>MTTVSEQANFTFSPEEVARFERDGYIGPVKIFEPEEMTRRWNIIRRQLLDRSLAIYPDSNGKANISNYDRHLDIDLLAEHIMRPEIVDRVGSLIGRNLLCWRSEFFPKYQGDEGTDWHQAATFAHATGKPQIIWPSDEGRPAFIGTITVWTAFTHSTEQNGCLQLMPGTHTSMNYDESKGMDYDADAINQREKDGIKRGFFGYDYRSLQKDPDWKPDESQAYPMVLKPGEAVI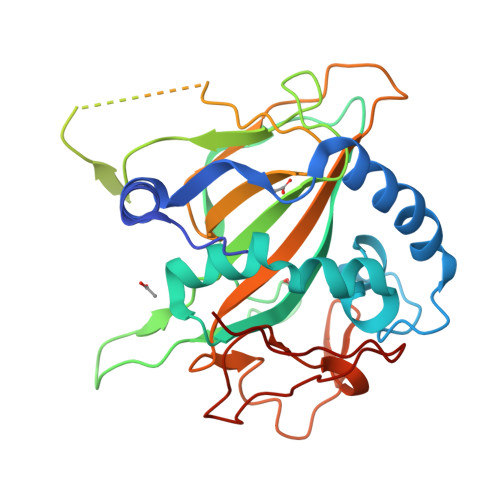FWSNTMHASLPHTGSKTDYRMGFAARYVPTQVQVYPGTENLTEYGDGINLEKYGAVLTSGVDEYGHNRIARTSQRGYEFVPRQIPS[2x]>[3x]QGMSKIFGIVNITTDSFSDGGLYLDTDKAIEHALHLVEDGADVIDLGAASSNPDTTEVGVVEE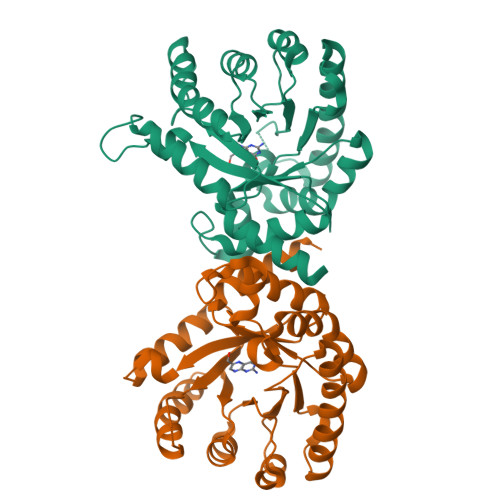IKRLKPVIKALKEKGISISVDTFKPEVQSFCIEQKVDFINDIQGFPYPEIYSGLAKSDCKLVLMHSVQRIGAATKVETNPEEVFTSMMEFFKERIAALVEAGVKRERIILDPGMGFFLGSNPETSILVLKRFPEIQEAFNLQVMIAVSRKSFLGKITGTDVKSRLAPTLAAEMYAYKKGADYLRTHDVKSLSDALKISKALG Nervous necrosis virus is a member of the family Nodaviridae that contains two genera: Alphanodavirus, which usually infects insects, and Betanodavirus, also known as piscine nodavirus. Virions of the Nodaviridae, including NNV, are non-enveloped, 25–30 nm in diameter and contain 180 copies of a single type of coat protein subunit arranged with T = 3 symmetry. The coat protein precursor self-assembles into T = 3 provirions. Provirions mature by spontaneous autocatalytic cleavage of the coat protein alpha post-assembly, producing proteins beta (38 kDa) and gamma (5 kDa) which remain part of the mature virion.

Here, we show that both transient expression of the coat protein of Atlantic cod nervous necrosis virus (ACNNV) in Nicotiana benthamiana leaves or in transgenic tobacco BY-2 cells leads to the production of VLPs. For a detailed structural analysis of the plant- produced ACNNV VLPs, cryo-EM was performed on the sample prepared from N. benthamiana leaves. Single-particle image processing was carried out in Relion, which allowed us to determine the solution structure of the VLP to a global resolution of 3.7 Å. The ACNNV VLP is an isometric particle with T = 3 symmetry, consistent with previously reported structures of the grouper nervous necrosis virus (GNNV) VLPs which share ∼85 % sequence identity. The shell domain displays the highest local resolution which allowed the building of an atomic model of the capsid shell. The viral asymmetric unit is composed of three quasi equivalent copies of the coat protein which have a characteristic jelly roll topology, with clear side-chain density. Three P-domains of the capsid protein interact and form spikes on the particle surface. The P-domains are attached to the rest of the capsid protein by a linker region and display lower local resolution, presumably as a result of flexibility. Overall, the cryo-EM analysis confirmed that the structure of the plant-produced VLPs is very similar that of material produced in other expression systems. When administered either intraperitoneally or intramuscularly to sea bass, the VLPs were shown to confer partial protection against subsequent challenge with ACNNV, indicating that plants can be used to produce effective vaccines for use in aquaculture.

>VRKGNKKLAKQATTKAVNPQPRRRNNNRRRGMRADAPLAKASTITGFGRGTNDVHLTGMSRIAQAVIPAGTGTDGYIVVDETIVPELLPRLGFAARIFQRYAVETLEFEIQPMCPANTGGGYVAGFLPDPTDSDHTFDAIQATRGAVVAKWWESRTIRPQYARALLWTSVGKEQRLTSPGRLILLCVGNNTDVVNVSVLCRWSVRLSVPSLETPEDTFAPILTLGPLYNDSLAANDFKSILLGSTQLDIAPEGAVYSLDRPLSIDYNLGTGDVDRAVYWHVKKVAGNAGTPAGWFHWGLWDNFNKTFTQGTAYYSDAQPRQILLPVGTLFTRADSGN[3x]>HHHHHIEGRHMAGPDRAELAELVRRLSVVHGRVTLSSGREADYYVDLRRATLHHRASALIGRLMRELTADWDYSVVGGLTLGADPVATAIMHAPGRPIDAFVVRKSAKAHGMQRLIEGSEVTGQRVLVVEDTSTTGNSALTAVHAVQDVGGEVVGVATVVDRATGAAEAIEAEGLRYRSVLGLADLGLD[4x]

The fifth step in the de novo biosynthetic pathway is catalyzed by the enzyme orotate phosphoribosyltransfrase that synthesises orotidine 5′-monophosphate (OMP) and pyrophosphate from α-D-5-phosphoribosyl-1-pyrophosphate (PRPP) and orotate (OA). Herein, we report the X-ray crystal structures of MtOPRT (coded by the rv0382c gene) in complex with PRPP, inorganic phosphate and an exogenous Fe(III) dicitrate molecule (ferric dicitrate, FDC) at 2.25 Å, 1.90 Å and 2.40 Å resolution, respectively. In all the structures herein described, both monomers composing the functional homodimeric unit are related by a 2-fold axis, with a solvent excluded surface between monomers of 1045 Å2 (13% of each subunit surface).

The inspection of the catalytic sites of the protein crystallized in absence of ligands revealed a bulky residual density located in the substrate-binding pocket I of one monomer of each of the two functional dimers present in the asymmetric unit. All efforts to unambiguously assigned such residual electron density to any of the substrates or products of the catalytic reaction proved unsuccessful. Given the predominant nature of the mononuclear dicitrate species at physiological conditions and the presence of iron(III) and citrate species in the crystallisation solution of ligand-free MtOPRT, we manually fitted the FDC molecule in the electron density with satisfactory results both in terms of ligand geometry and refinement statistics. However, both approaches gave unsatisfactory results, poor fitting scores (CC < 0.7) and refinement statistics, prompting us to conclude that a mononuclear iron dicitrate is present in the MtOPRT active site. FDC is held in place by hydrogen bonds involving the non-conserved Ala99 (3.5 Å, long range H-bond). These interactions contribute to the stabilisation of the “flexible loop” of the neighbouring chain. Moreover, FDC O7(2) interacts with the amidic N- and O-atoms of Thr124 (3.1 Å and 3.2 Å, respectively), while the Oγ of the conserved Ser26 forms hydrogen bond with O1(2) of FDC (3.3 Å). Noteworthy, in our MtOPRT structure, the conserved Ser26 is shown to exclusively interact with the FDC molecule, and does not participate in either OA, OMP or PRPP binding in MtOPRT orthologs. Moreover, in order to further support the structural data, we performed thermal shift experiments that showed a stabilizing effect of FDC, not matched by either Fe(III) or citrate alone, with a KD of 1.6 mM, well below the concentration of Fe(III)-citrate present in the crystallization buffer.N-(4-carbamimidamidobutyl)ethanamide 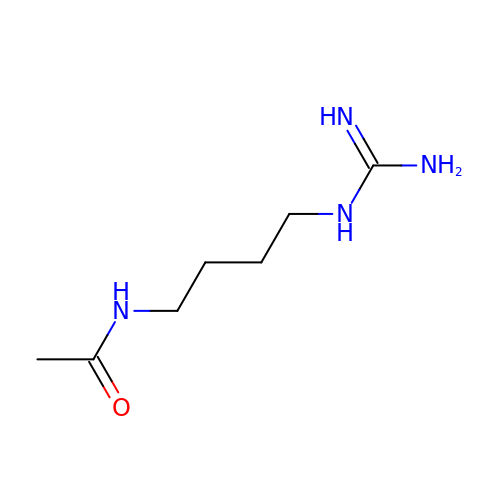| C7 H16 N4 O | JMACEDIUUMWDIC-UHFFFAOYSA-N3-[(4-chloro-3-methoxyphenyl)amino]-1-[(3R,4S)-4-cyanooxan-3-yl]-1H-pyrazole-4-carboxamide 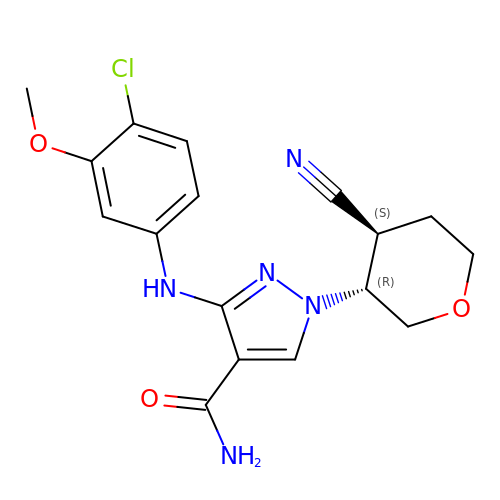| C17 H18 Cl N5 O3 | MFWQXZZXOUIDTN-YGRLFVJLSA-N>SHFNPLSLEELGSNTGIQVFNQIVKSRPHDNIVISPHGIASVLGMLQLGADGRTKKQLAMVMRYGVNGVGKILKKINKAIVSKKNKDIVTVANAVFVKNASEIEVPFVTRNKDVFQCEVRNVNFEDPASACDSINAWVKNETRDMIDNLLSPDLIDGVLTRLVLVNAVYFKGLWKSRFQPENTKKRTFVAADGKSYQVPMLAQLSVFRCGSTSAPNDLWYNFIELPYHGESISMLIALPTESSTPLSAIIPHISTKTIDSWMSIMVPKRVQVILPKFTAVAQTDLKEPLKVLGITDMFDSSKANFAKITTGSENLHVSHILQKAKIEVSEDGTKASAATTAIL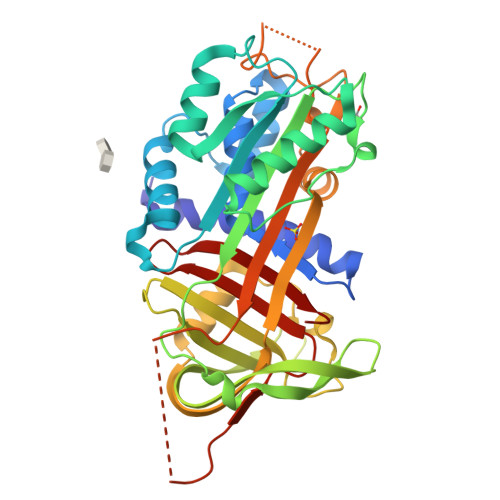IARSSPPWFIVDRPFLFFIRHNPTGAVLFMGQINKP[2x]Herein, we describe the use of GE to optimize a fragment‐derived inhibitor of Mycobacterium tuberculosis pantothenate synthetase, an attractive target for developing new drugs against tuberculosis. Pantothenate synthetase catalyzes the ATP‐dependent formation of an amide bond between pantoate and β‐alanine. The work presented here demonstrates the use of GE analysis to critically and thoroughly examine the binding distribution of a lead compound and illustrates the practicality of applying GE analysis to modify parts of a molecule that are not making efficient contributions to binding. In this case, it led to the generation of a relatively potent and bactericidal inhibitor of M. tuberculosis pantothenate synthetase.

Based on these observations, the initial optimization strategy was focused on replacement of the methyl pyridine and the benzofuran groups rather than the acyl sulfonamide linker in both compounds 5 and 8. Compounds were designed with the objective of optimizing interactions at the P1 or P2 sites of panthothenate synthetase. Consequently, 1‐ethyl‐3‐(3‐dimethylaminopropyl)‐carbodiimide (EDCI)‐mediated coupling reactions were employed to generate a series of indole acyl sulfonamide compounds (10–19; the syntheses are described in the Supporting Information).

>[2x]MAIPAFHPGELNVYSAPGDVADVSRALRLTGRRVMLVPTMGALHEGHLALVRAAKRVPGSVVVVSIFVNPMQFGAGGDLDAYPRTPDDDLAQLRAEGVEIAFTPTTAAMYPDGLRTTVQPGPLAAELEGGPRPTHFAGVLTVVLKLLQIVRPDRVFFGEKDYQQLVLIRQLVADFNLDVAVVGVPTVREADGLAMSSRNRYLDPAQRAAAVALSAALTAAAHAATAGAQAALDAARAVLDAAPGVAVDYLELRDIGLGPMPLNGSGRLLVAARLGTTRLLDNIAIEIGTFAGTDRPDGYR>MEEPEEPADSGQSLVPVYIYSPEYVSMCDSLAKIPKRASMVHSLIEAYALHKQMRIVKPKVASMEEMATFHTDAYLQHLQKVSQEGDDDHPDSIEYGLGYDCPATEGIFDYAAAIGGATITAAQCLIDGMCKVAINWSGGWHHAKKDEASGFCYLNDAVLGILRLRRKFERILYVDLDLHHGDGVEDAFSFTSKVMTVSLHKFSPGFFPGTGDVSDVGLGKGRYYSVNVPIQDGIQDEKYYQICESVLKEVYQAFNPKAVVLQLGADTIAGDPMCSFNMTPVGIGKCLKYILQWQLATLILGGGGYNLANMARCWTYLTGVILGKTLSSEIPDHEFFTAYGPDYVLEITPSCRPDRNEPHRIQQILN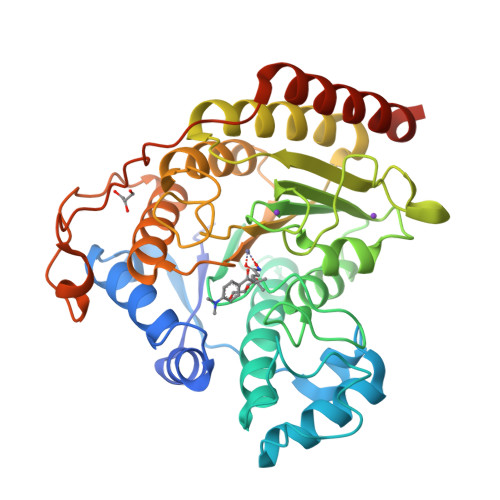YIKGNLKHVVIEGRGSHHHHHH[2x]> RKMFRALMPALEELTFDPSSAHPSLVVSSSGRRVECSEQKAPPAGEDPRQFDKAVAVVAHQQLSEGEHYWEVDVGDKPRWALGVIA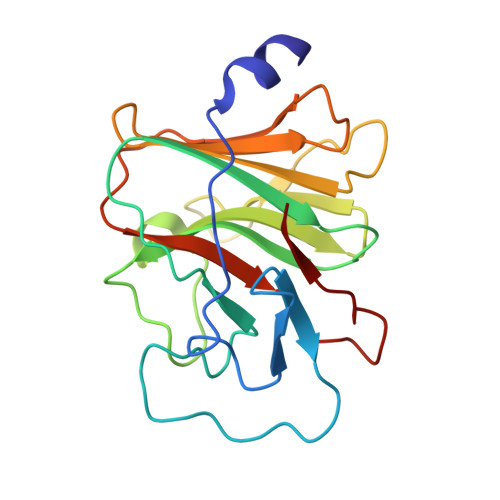AEAPRRGRLHAVPSQGLWLLGLREGKILEAHVEAKEPRALRSPERRPTRIGLYLSFGDGVLSFYDASDADALVPLFAFHERLPRPVYPFFDVCWHDKGKNAQPLLLV>MSSSHHHHHHMPTKKQKSKSKLKPFFALVRRTNPSYGKLAFALALSVVTTLVSLLIPLLTKQLVDGFSMSNLSGTQIGLIALVFFVQAGLSAYATYALNYNGQKIISGLRELLWKKLIKLPVSYFDTNASGETVSRVTNDTMVVKELITTHISGFITGIISVIGSLTILFIMNWKLTLLVLVVVPLAALILVPIGRKMFSISRETQDETARFTGLLNQILPEIRLVKASNAEDVEYGRGKMGISSLFKLGVREAKVQSLVGPLISLVLMAALVAVIGYGGMQVSSGELTAGALVAFILYLFQIIMPMGQITTFFTQLQKSIGATERMIEILAEEEEDTVTGKQIENAHLPIQLDRVSFGYKPDQLILKEVSAVIEAGKVTAIVGPSGGGKTTLFKLLERFYSPTAGTIRLGDEPVDTYSLESWREHIGYVSQESPLMSGTIRENICYGLERDVTDAEIEKAAEMAYALNFIK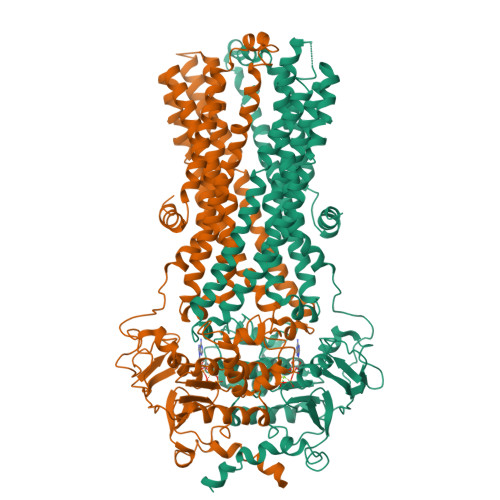ELPNQFDTEVGERGIMLSGGQRQRIAIARALLRNPSILMLDAATSSLDSQSEKSVQQALEVLMEGRTTIVIAHRLSTVVDADQLLFVEKGEITGRGTHHELMASHGLYRDFAEQQLKMNADLENKAG[4x]4-[(but-2-yn-1-yl)(methyl)amino]-1lambda~6~-thiane-1,1-dione 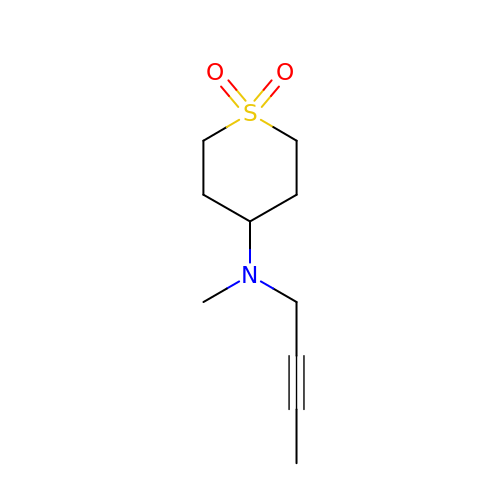| C10 H17 N O2 S | PFUSCIQPWKGDKP-UHFFFAOYSA-N>GSVYMLFIDIEVNGVPIKAFVDSGAQSTFMSYACAQKCSLLRLMDTRYRGVAQGVGKTEIVGKIHLATLKIGQRFFPSSFTVLQDNKVEFLFGLDLLRRYQCCIDLKKSVLRIDNEEIPFLSEKDITK[12x]

Ddi1 is a multidomain protein that belongs to the ubiquitin receptor family of proteins. The Ddi1 proteins contain a highly conserved retroviral protease (RVP)-like domain along with other domains. The crystal structures of the RVP domains of Ddi1 from T. gondii and C. hominis were determined; they form homodimers similar to those observed in HIV protease and the reported structures of the same domain from Saccharomyces cerevisiae, Leishmania major and humans. The ubiquitin receptor family of proteins bind to ubiquitinated substrates through the UBA domain and deliver the substrates to the proteasome by interacting with the regulatory subunit of the 26S proteasome through the UBL domain.

The solution had six dimers in the asymmetric unit (ASU) with TFZ and LLG of 35 and 3173, respectively, in the space group P41212. Out of the six dimers in the ASU, the flap regions of both the subunits in only one dimer and the flaps of three other subunits in different dimers had electron density. In the ToxoDdi1-RVP structure, a hydrophobic binding cavity is formed by the side chains of residues Met398, Ph305, Phe313, Ala318, Phe322, Ile353, Thr374, Leu376, Val381 and Leu384. The binding cavity in the ToxoDdi1-RVP structure has a width of ∼27 ​Å (distance between the Cα atoms of Asn379 residues of the two subunits of the dimer), while in the CrypDdi1-RVP structure, the cavity width is ∼22.5 ​Å (distance between the Cα atoms of Ser284 of the two subunits). The cavity in ToxoDdi1-RVP is larger than that formed in HIV protease which has a width of ∼19–22 ​Å in the open form, while the size of the cavity in CrypDdi1-RVP is comparable to that of HIV protease. The flap of ToxoDdi1-RVP forms a loop without the characteristic β-hairpin structure. The distance between the Cα atoms of Val348 residues located at the tips of the two flaps is 11.5 ​Å. The distance between the Cα atom of Val348 and the Cα atom of Asp315 (catalytic aspartate) is 21.6 ​Å in one subunit and 21.2 ​Å in the other. The MD simulations showed that RMSD values of the flaps of subunits A and B stabilized at about 5.5 and 6.5 ​Å, respectively. Of all the inhibitors tested, nelfinavir showed binding to ToxoDdi1-RVP with a Kd of 237.6 ​± ​6.3 ​μM and saquinavir showed binding to CrypDdi1-RVP with a Kd of 242.1 ​± ​3 ​μM.>MAIKKTTEIDAILLNLNKAIDAHYQWLVSMFHSVVARDASKPEITDNHSYGLCQFGRWIDHL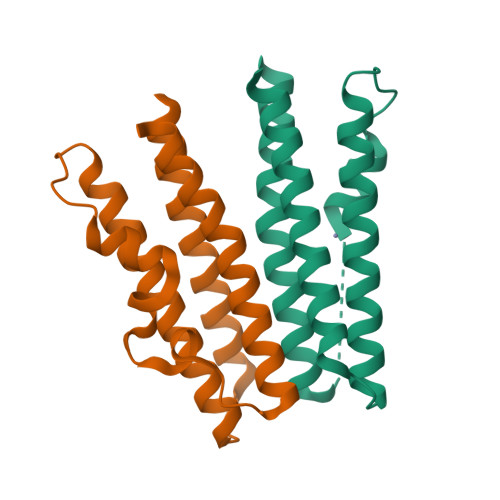GPLDNDELPYVRLMDSAHQHMHNCGRELMLAIVENHWQDAHFDAFQEGLLSFTAALTDYKIYLLTLEHHHHHH[2x]>[2x]TDKERFIASLMARMSNAEKIGQLRLVSVGADHPKEALMADIRAGKVGAIFNTVTRPDIRAMQDQVRHSRLKIPLFHAYDVAHGHRTIFPISLGLAASWDPEVVARSARISALEASADGLDMSFSPMVDITRDARWGRVSEGFGEDTYLTSLLSGVMVRAYQGSNLAAPDSIMAAVKHFALYGAAEGGRDYNTVDMSLPRMFQDYLPPYKAAVDAGAGAVMVSLNTINGVPATANRWLLTDLLRQQWGFKGLTISNHGAVKELIKHGLAGNERDATRLAIQAGVDMNMN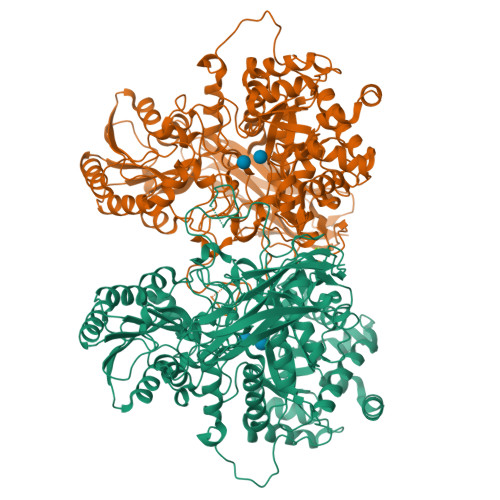DDLYSTWLPKLLAAGEIDQADIDRACRDVLAAKYDLGLFADPYRRLGKPDDPPFDTNAESRLHRQAAREVAREGLVLLKNRDGLLPLKKQGRIAVIGPLAKSQRDVIGSWSAAGVPRQAVTVYQGLANAVGERATLLYAKGANVSGDQAILDYLNSYNPEVEVDPRSAEAMLEEALRTARDADLVVAVVGESQGMAHEASSRTDLRIPASQRRLLKALKATGKPLVLVLMNGRPLSLGWEQENADAILETWFSGTEGGNAIADVLFGEHNPSGKLTMSFPRSVGQVPVYYNHLNTGRPMDHDNPGKYTSRYFDEANGPLYPFGYGLSYTEFSLSPLRLSSERLARGATLEARVTLSNSGKRAGATVVQLYLQDPVASLSRPVKELRGFRKVMLEPGESREIVFRLGEADLKFYDSQLRHTAEPGEFKVFVGLDSAQTESRSFTLL>MDLKIKNKVCIITGGAKGIGYGIAKLWASEGGIPVIFSRSMPKEHDKELKKLSSEYEFYEIDLKNYEQIEKLVKKVAIKHGGIYALVNNAGTNDNLHIENTSTQDLIKSYENNLFHYYTMTKECLPYIKKEQGSILNIVSKTGITGQGRTSAYASAKAAQMGFTREWACAFAKDNVRVNAIAPAEVMTPLYEKWLQNFPNPKEQYEKIAKAIPLGHRFTTIEEIANTAVFTLSPLASHTTGQILMPDGGYVHLDRALNWDENTRGHHHHHH[4x]

We also characterize the putative dehydrogenase Cj0485 through crystallography, enzymology, and multiple biological assays to confirm its function as a fucose dehydrogenase, which we have named FucX. Several aldose sugars in both d- and l-configurations were screened as substrates and Cj0485 displayed substantial activity on l-fucose and d-arabinose and with low levels of activity on l-galactose. The Cj0485 monomer adopts a Rossmann-like fold comprising a central seven-stranded twisted β-sheet sandwiched between two trios of parallel α-helices. The holo-enzyme’s asymmetric unit contained four monomers that were arranged as tetramers with identical D2 symmetry to the crystallographic tetramer observed in the apo-complex. PISA31 analysis predicts this recurring tetramer to be a stable conformation, supporting the likelihood that the tetramer is the biologically relevant assembly of the enzyme.

To provide insight into the substrate specificity of Cj0485, we solved X-ray crystal structures of this enzyme alone and in complex with NADP+. The holo-enzyme in complex with NADP+ also crystallized in the space group P1. Kinetic analysis of Cj0485 activity using an excess of l-fucose as a substrate revealed a preference for NADP+ as a cofactor with KM, kcat, and kcat/KM values of 9.9 ± 1.9 μM, 16.5 ± 0.7 s−1 and 1.7 ± 0.3 μM−1 s−1, respectively compared with KM, kcat, and kcat/KM values of 6050 ± 1080 μM, 20.5 ± 2.1 s−1 and 0.0034 ± 0.0008 μM−1 s−1, respectively, for NAD+. Though we attempted extensive co-crystallization and soaking experiments, we were unable to obtain a ternary complex of Cj0485, NADP+ and l-fucose. However, comparison of our NADP+ complex to the ternary complex of FabG revealed insight into substrate specificity. Despite only 45% amino acid sequence identity, the NADP+ and l-fucose binding sites are comprised of identical amino acid side chains, pointing to indistinguishable modes of substrate accommodation and consistent with the matching specificities of the two enzymes. The only notable difference, likely owing to the lack of bound fucose in Cj0485, was the more open conformation of the catalytic site in Cj0485 whereby an α-helical “lid” enclosing the l-fucose binding site was retracted by ~5.8 Å relative to its conformation in FabG. The apparent selectivity of these enzymes for β-l-fucose may result from van der Waals interactions between the enzyme active site and the C6 methyl group of this sugar, leading to a higher binding affinity compared with d-arabinose, which lacks the C6 methyl group.> XELKAIAQEFKAIAKEFKA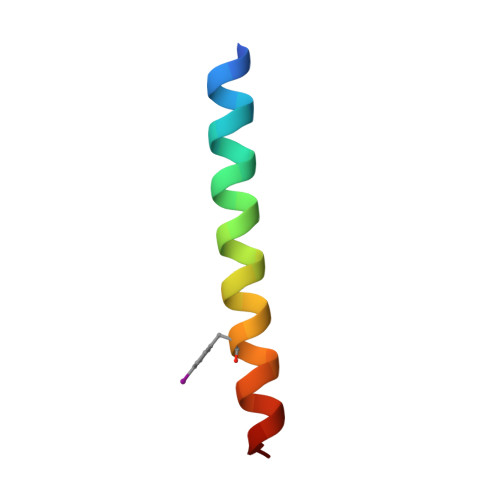IAFEFKAIAQKX4-ANDROSTENE-3-17-DIONE 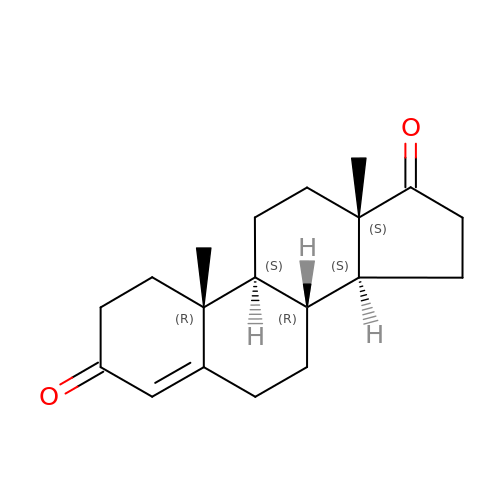| C19 H26 O2 | AEMFNILZOJDQLW-QAGGRKNESA-N> SGISLDNSYKMDYPEMGLCIIINNKNFHKSTGMTSRSGTDVDAANLRETFRNLKYEVRNKNDLTREEIVELMRDV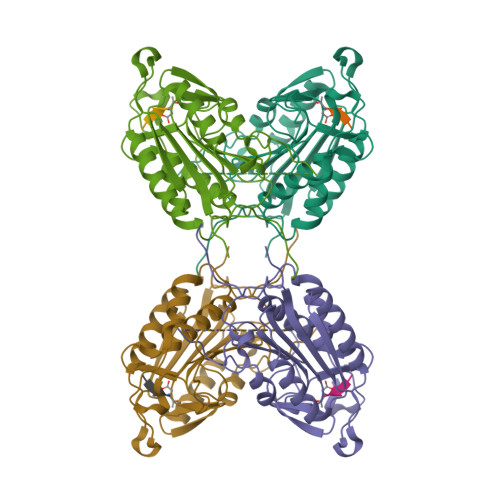SKEDHSKRSSFVCVLLSHGEEGIIFGTNGPVDLKKITNFFRGDRCRSLTGKPKLFIIQACRGTELDCGIETDSGVDDDMACHKIPVEADFLYAYSTAPGYYSWRNSKDGSWFIQSLCAMLKQYADKLEFMHILTRVNRKVATEFESFSFDATFHAKKQIPCIESMLTKELYFYHA>[2x]MDLSTSINPWFVTGFTDAEGSFMIHLEKNKDKWRVRPTFQIKLDIRDKSLLEEIKNYFNNTGSINTSNKECVYKVRSLKDISIIISHFDKYNLITQKKADFELFKKIINKLNSQEHLSYEVGATVLQEIISIRASMNLGLSSSVKEDFPHIIPSNRPLIENMNIPHPEWMAGFVSG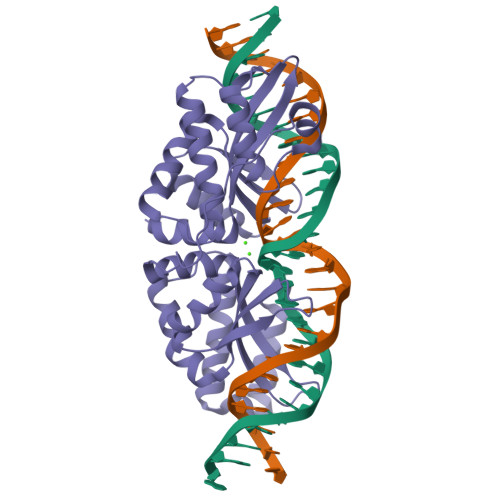EGSFSVYTTSDDKYVSLSFRVSQHNKDKQLLKSFVDFFGCGGFNYHNKGNKAVIFVTRKFEDINDKIIPLFNEYKIKGVKYKDFKDWSKVAKMIESKSHLTTNGYKEICKIKENMNSYRKSSVN> GSPSVRTMYTREELLRIATLASAMDL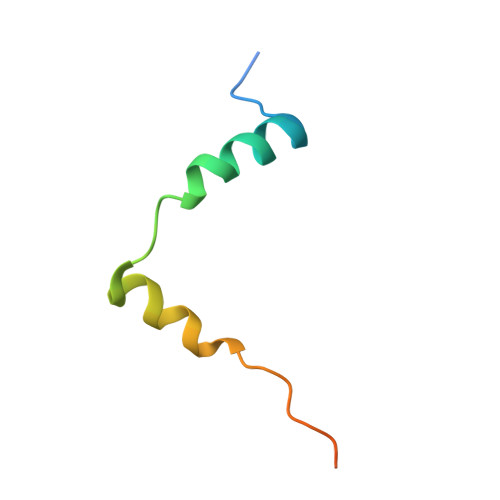GPEVLRKFDVIEVAEPVPTPKRRDAES>CGCCAGCG[2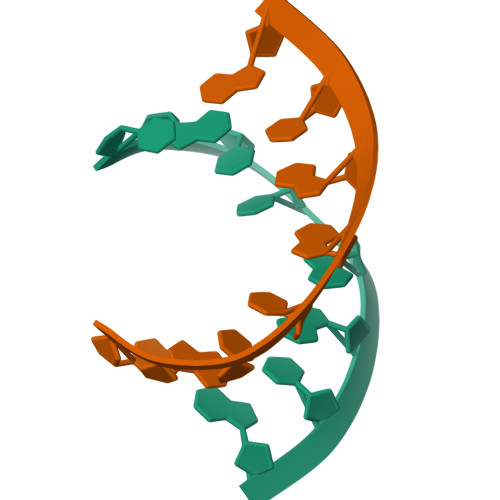x]>GSSSSLPLYNQQVGDCCIIRVSLDVDNGNMYKSILVTSQDKAPTVIRKAMDKHNLDEDEPEDYELLQIISE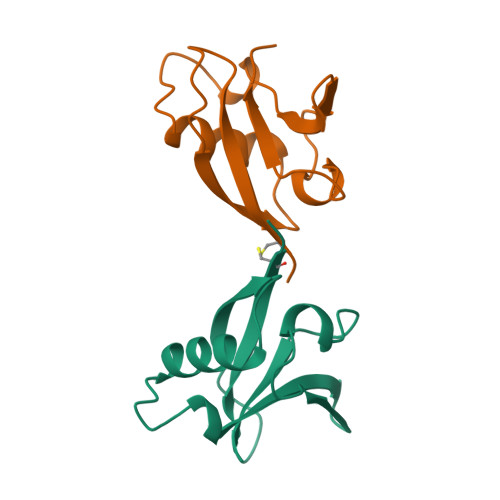DHKLKIPENANVFYAMNSAANYDFILKKR[2x]> LGTDDDDKMKHYSIQPANLEFNAEGTPVSRDFDDVYFSNDNGLEETRYVFLGGNQLEVRFPEHPHPLFVVAESGFGTGLNFLTLWQAFDQFREAHPQAQLQRLHFISFEKFPLTRADLALAHQHWPELAPWAEQLQAQWPMPLPGCHRLLLDAGRVTLDLWFGDINELTSQLDDSLNQKVDAWFLDGFAPAKNPDMWTQNLFNAMARLARPGGTLATFTSAGFVRRGLQDAGFTMQKRKGFGRKREMLCGVMEQTLPLPCSAPWFNRTG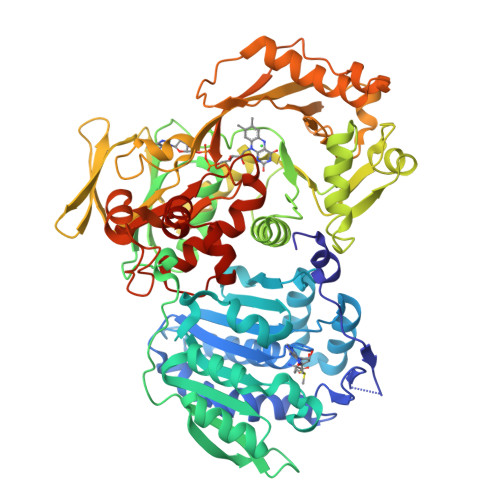SSKREAAIIGGGIASALLSLALLRRGWQVTLYCADEAPALGASGNRQGALYPLLSKHDEALNRFFSNAFTFARRFYDQLPVKFDHDWCGVTQLGWDEKSQHKIAQMLSMDLPAELAVAVEANAVEQITGVATNCSGITYPQGGWLCPAELTRNVLELAQQQGLQIYYQYQLQNFSRKDDCWLLNFAGDQQATHSVVVLANGHQISRFSQTSTLPVYSVAGQVSHIPTTPELAELKQVLCYDGYLTPQNPANQHHCIGASYHRGSEDTAYSEDDQQQNRQRLIDCFPQAQWAKEVDVSDKEARCGVRCATRDHLPMVGNVPDYEATLVEYASLAEQKDEAVSAPVFDDLFMFAALGSRGLCSAPLCAEILAAQMSDEPIPMDASTLAALNPNRLWVRKLLKGKAVKAG>MKFTVEREHLLKPLQQVSGPLGGRPTLPILGNLLLQVADGTLSLTGTDLEMEMVARVALVQPHEPGATTVPARKFFDICRGLPEGAEIAVQLEGERMLVRSGRSRFSLSTLPAADFPNLDDWQSEVEFTLPQATMKRLIEATQFSMAHQDVRYYLNGMLFETEGEELRTVATDGHRLAVCSMPIGQSLPSHSVIVPRKGVIELMRMLDGGDNPLRVQIGSNNIRAHVGDFIFTSKLVDGRFPDYRRVLPKNPDKHLEAGCDLLKQAFARAAILSNEKFRGVRLYVSENQLKITANNPEQEEAEEILDVTYSGAEMEIGFNVSYVLDVLNALKCENVRMM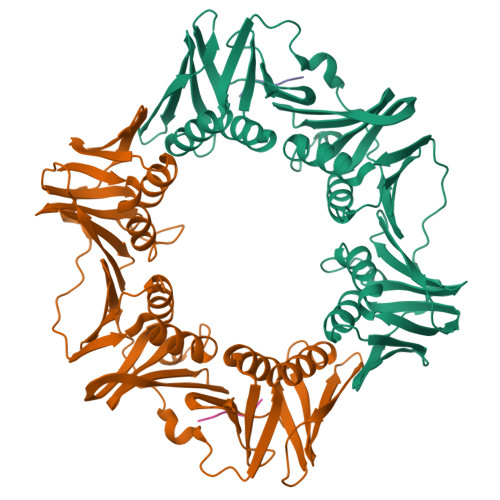LTDSVSSVQIEDAASQSAAYVVMPMRL[6x];>[5x]XQLDLF>[12x]SSFHATTIFAVQHKGRSAMSGDGQVTFGQAVVMKHTARKVRKLFNGKVLAGFAGSVADAFTLFEKFEAKLEEYNGNLKRAAVELAKEWRSDKVLRKLEAMLIVMNQDTL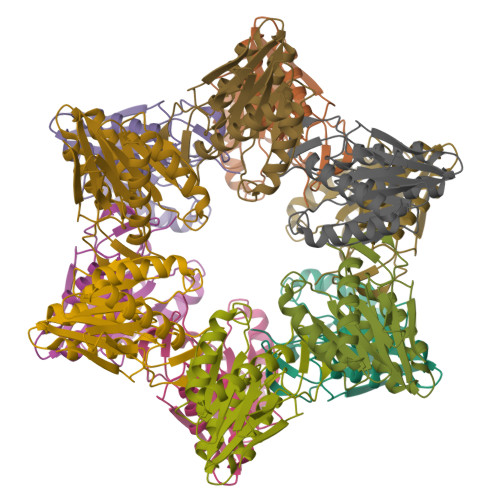LLVSGTGEVIEPDDGILAIGSGGNYALAAGRALKKHAGESMSASEIARAALETAGEICVYTNDQIILEELE>[2x]SHHHHHHSSSENLYFQRGYAGEITAAVALDTVVNDPSAVLIDVRAAREKEASGVPDVPGAASSKVLEVEFAALED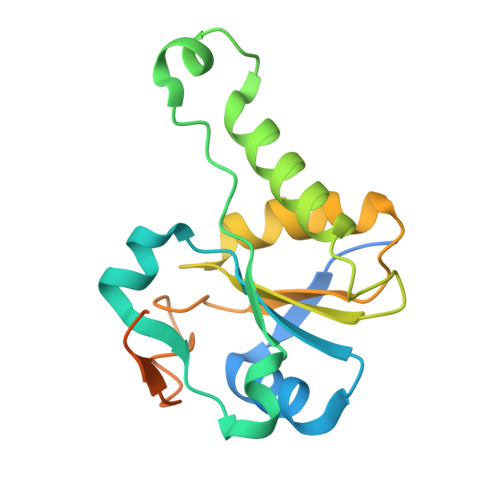KKLRSQLKDPSFIEAQTTALQIASLRRIGTGSKVILLDRYGPQAEAVARELAKKGYSRVYVVTGGFDGRAGWIQSKLQIKPFTATNLTFAAPAFGARTGTTSTRRLPAPRA> HIRGSITQGIPRSY;> AFTTGLVYDTLMLKHQCTCGSSSSHPEHAGRIQSIWSRLQETGLRGKCECIRGRKATLEELQTVHSEAHTLLYGTNPLNRQKLDSKKLLGSLASVFVRLPCGGVGVDSDTIWNEVHSAGAARLAVGCVVELVFKVATGELKNGFAVVRPPGHHAEESTPMGFCYFNSVAVAAKLLQQRLSVSKILIVDWDVHHGNGTQQAFYSDPSVLYMSLHRYDDGNFFPGSGAPDEVGTGPGVGFNVNMAFTGGLDPPMGDAEYLAAFRTVVMPIASEFAPDVVLVSSGFDAVEGHPTPLGGYNLSARCFGYLTKQLMGLAGGRIVLALEGGYDLTAICDASEACVSALLGNELDPLPEKVLQQRPNANAV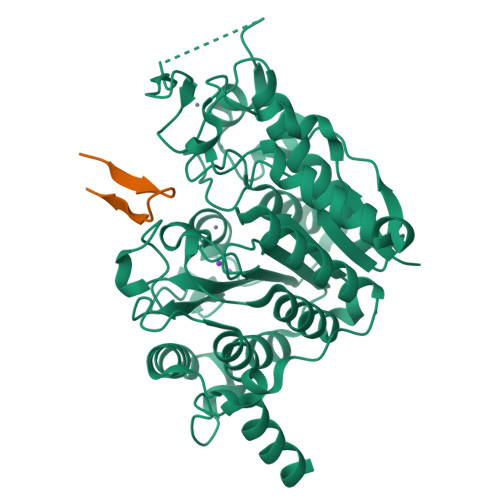RSMEKVMEIHSKYWRCLQRTTSTAGRSLIEAQTCENEEA> CKGADGAHGVNGCPGTAGAAGSVGGPGCDGGHGGNGGNGNPGCAGGVGGAGGASG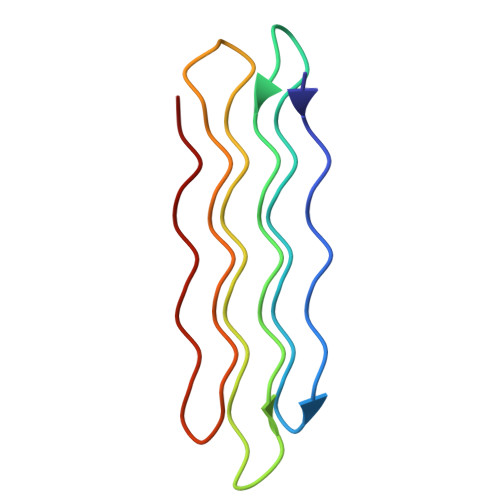GTGVGGRGGKGGSGTPKGADGAPGAP>GSENLYFQSGSMARQERAIRTRQTILVAAAEVFDEVGYEAATISDVLKRSGVTKGALYFHFTSKQELAQAVLAEQVASLPRVPEQELKLQQSLDEALLLAHLLREGTGDPIVQGSVRLTVDQGSPRDHLNRRVPMQAWTEHTQSLFEEARAKGEILPHADVEALAKLFVGAFTGVQVLSRIMTGRADLAERVADLYRHLMPSFAMPGILVRLDFSPERGSRVYEAAMKQRESAAASTTDAARTLE[8x]

We also present structures of AvaR1, in isolation (2.4 Å resolution), in complex with avenolide (2.0 Å resolution), and bound to a synthetic DNA oligonucleotide (3.09 Å resolution) derived from its natural binding site. The overall structure is reminiscent of that of other TetR-family transcriptional repressors, and consists of an obligate homodimer. Each monomer is entirely helical and consists of a DNA-binding domain (DBD; composed of α helices 1–4), and a ligand-binding domain (LBD; consisting of α helices 5–13). The dimer interface is formed via interactions between the two LBDs and is formed mainly through hydrophobic packing interactions.

In order to gain further insights into the mechanism of hormone-mediated de-repression, we also determined the structure of AvaR1 bound to a synthetic oligonucleotide derived from the autoregulator responsive element (ARE) sequence. DNase foot-printing analysis had previously established the identity of the ARE located upstream of the aco gene, but this response element is pseudopalindromic. Crystallization efforts with the symmetric AvaR1 homodimer yielded crystals that did not diffract beyond 8 Å, presumably as a result of the asymmetry of the ARE operator. Efforts using an artificial palindromic sequence derived by inverting and repeating each half of the pseudo palindrome yielded crystals that diffracted to 3.09 Å resolution, and the structure was determined by molecular replacement. As a result of the use of this symmetric DNA, each homodimer in the crystallographic asymmetric unit is bound to a monomer from an adjacent ARE. The structure shows that each DBD interacts with one half of the palindrome of the DNA duplex. Numerous contacts are formed between helix α1 of the DBD and the duplex, including Arg5, which inserts into the major groove and interacts with Thy7, as well as between Lys43 and Ade15 of the ARE. Additional non-specific interactions include those between Thr10, Thr42, and Tyr47 and the backbone phosphate of the duplex. A comparison of the ligand-binding sites with that in the hormone-bound structure reveals that the binding pocket is further occluded through movements of Trp127 and the loop harboring Gln64, consistent with the roles of these residues in effecting conformational movements of the DBD upon binding of the hormone.>[5x]GGVEVLEVKTGVDAITEVECFLNPEMGDPDENLRGFSLKLSAANDFSSDSPERKMLPCYSTARIPLPNLNEDLTSGNLLMWEAVTVQTEVIGITSMLNLHAGSQKVHEHGGGKPIQGSNFHFFAVGGEPLEMQGVLMNYRSKYPDGTITPKNPTAQSQVMNTDHKAYLDKNNAYPVECWVPDPSRNENARYFGTFTGGENVPPVLHVTNTATT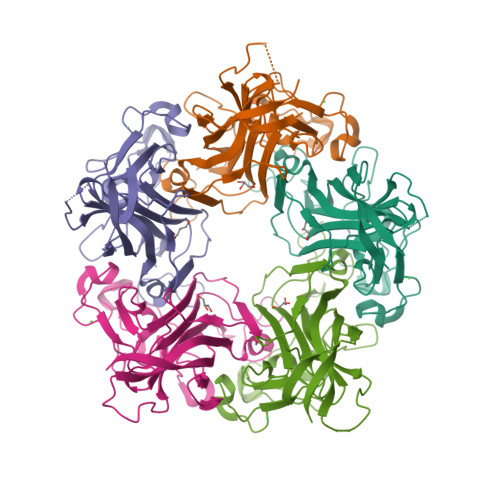VLLDEQGVGPLCKADSLYVSAADICGLFTNSSGTQQWRGLARYFKIRLRKRSVKNPYP(2~{R})-4-[[(2~{R},3~{S},4~{R},5~{R})-5-(6-aminopurin-9-yl)-3,4-bis(oxidanyl)oxolan-2-yl]methyl-[[4-azanyl-1-(methoxymethyl)-2-oxidanylidene-pyrimidin-5-yl]methyl]amino]-2-azanyl-butanoic 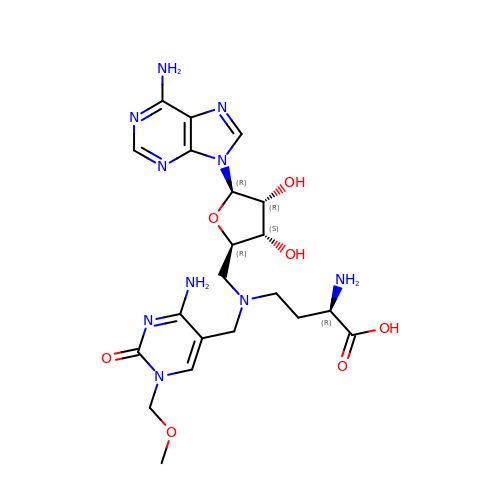acid | C21 H30 N10 O7 | UCWJYOSDGSOMTM-FSVZYJJUSA-N> LIPVSLVDLININIIFY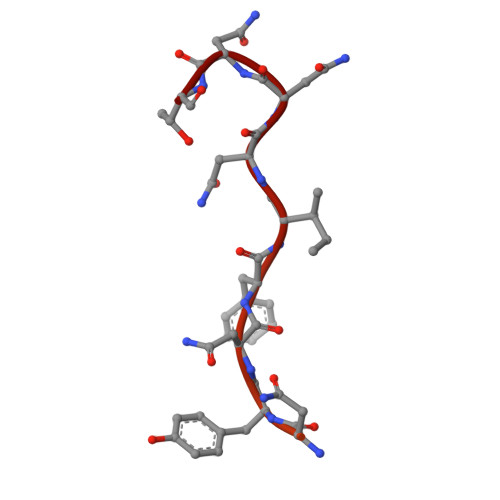ILLLYTLLLFFIPLFLASINYTYHYIYKYYNYNYNFINNNT> GALIEEVFADAFDNEYIRAMEDAALLFGNITLTTDSFTVKPLFFPGGDIGKLAVCGTVNDA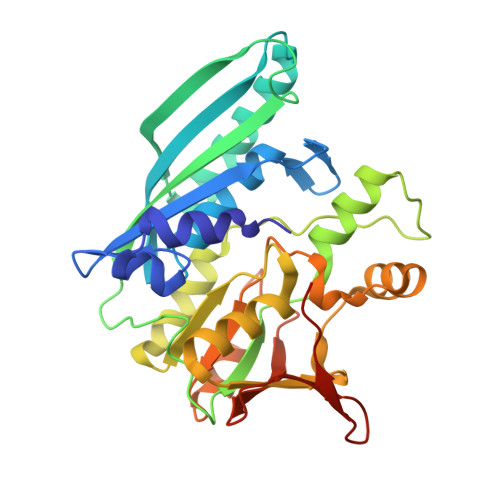SMRGAKPLFLTAAFIIEEGFPVEDLKKIVKSMAEAAKEAGVKIVAGDTKVVEKGSVDRIFINTSGIGVLYEGANVSIKNAKPGDIVLISGTIGDHGMAVMSAREELQFDTPIFSDVAPLNGLIEKLMTLGEAIKVLRDPTRGGVAEVLYEISKMSGVGIKIYEEKLPVKESVKSACEFMGIDFLHLANEGKVVVVVERDYAEKALEIMKSHEYGKDAEIIGEVNDSKLVTINTIYGTSRIVDRPIGELLPRIC>[2x]SNAMSGNGNAAATAEENSPKM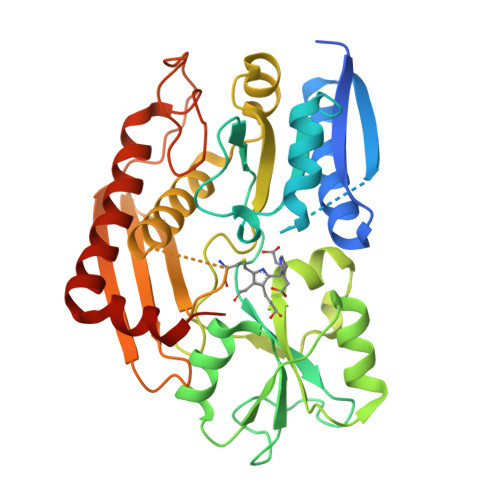RVIRVGTRKSQLARIQTDSVVATLKASYPGLQFEIIAMSTTGDKILDTALSKIGEKSLFTKELEHALEKNEVDLVVHSLKDLPTVLPPGFTIGAICKRENPHDAVVFHPKFVGKTLETLPEKSVVGTSSLRRAAQLQRKFPHLEFRSIRGNLNTRLRKLDEQQEFSAIILATAGLQRMGWHNRVGQILHPEECMYAVGQGALGVEVRAKDQDILDLVGVLHDPETLLRCIAERAFLRHLEGGCSVPVAVHTAMKDGQLYLTGGVWSLDGSDSIQETMQATIHVPAQHEDGPEDDPQLVGITARNIPRGPQLAAQNLGISLANLLLSKGAKNILDVARQLNDAH> MHHHHHHMLEAKFEEASLFKRIIDGFKDCVQLVNFQCKEDGIIAQAVDDSRVLLVSLEIGVEAFQEYACAHPVTL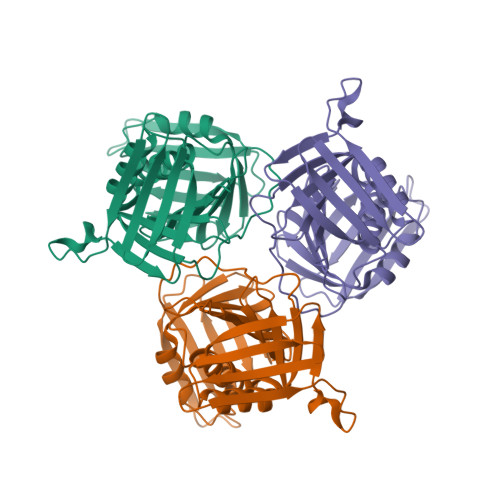GMDLTSLSKILRCGNNTDTLTLIADNTPDSIILLFEDTKKDRIAEYSLKLMDIDADFLKIEELQYDSTLSLPSSEFSKIVRDLSQLSDSINIMITKETIKFVADGDIGSGSVIIKPFVDMEHPETSIKLEMDQPVDLTFGAKYLLDIIKGSSLSDRVGIRLSSEAPALFQFDLKSGFLQFFLAPKFNDEE(3R)-3-(5-fluoro-1H-indol-3-yl)pyrrolidine-2,5-dione | C12 H9 F N2 O2 | 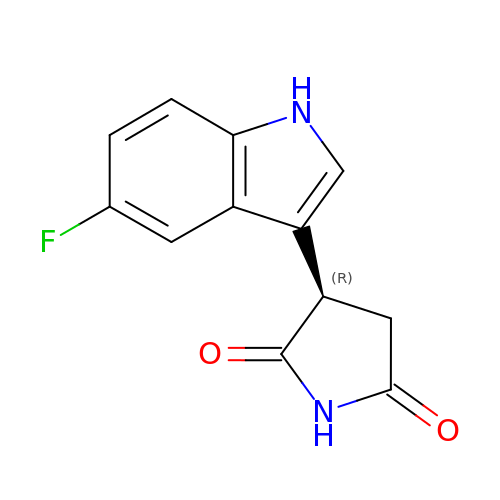MXKLDYKORJEOPR-MRVPVSSYSA-N> VVGGTEAQRNSWPSQISLQYRSGSSWAHTCGGTLIRQNWVMTAAHCVDRELTFRVVVGEHNLNQNNGTEQYVGVQKIVVHPYWNTDDVAAGYDIALLRLAQSVTLNSYVQLGVLPRAGTILANNSPCYITGWGLTRTNGQLAQTLQQAYLPTVDYAICSSSSYWGSTVKNSMVCAGGDGVRSGCQGDSGGPLHCLVNGQYAVHGVTSFVSR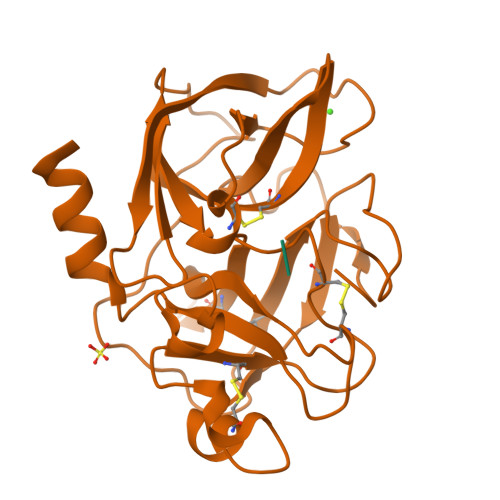LGCNVTRKPTVFTRVSAYISWINNVIASN;> NPIAA> FVLLIGAAFATEDDKIVGGYECKAYSQAHQVSLNSGYHFCGGSLVNENWVVSAAHCYKSRVEVRLGEHNIKVTEGSEQFISSSRVIRHPNYSSYNIDNDIMLIKLSKPATLNTYVQPVALPTSCAPAGTMCTVSGWGNTMSSTADSNKLQCLNIPILSYSDCNNSYPGMITNAMFC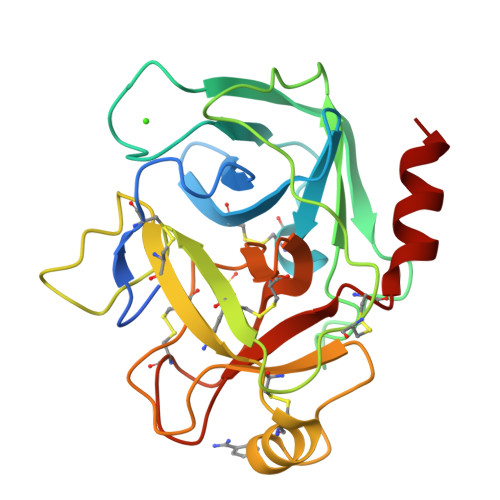AGYLEGGKDSCQGDSGGPVVCNGELQGVVSWGYGCAEPGNPGVYAKVCIFNDWLTSTMASY>[4x]GKAFDDGAFTGIREINLSYNKETAIGDFQVVYDLNGSPYVGQNHKSFITGFTPVKISLDFPSEYIMEVSGYTGNVSGYVVVRSLTFKTNKKTYGPY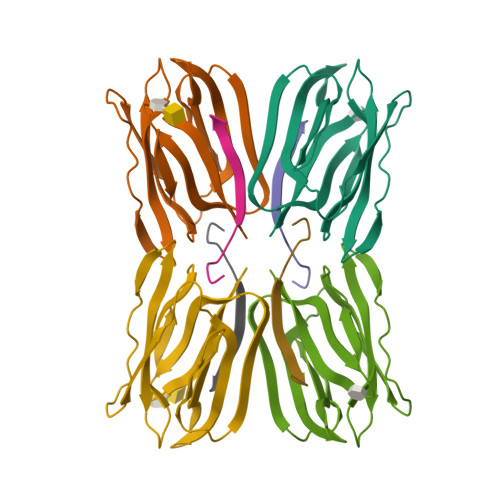GVTSGTPFNLPIENGLIVGFKGSIGYWLDYFSMYLSL;>[4x]DEQSGKSQTVIVGPWGAKVS> MASEVMNLSEEDIQFCQKAFSDYDEDGLGAIKVSDLKLALENIGCSLSENDLFKMISEVDEKNTGLIKFSDFLNIYYKQKYANLGDDDQDLVDAFVAMGGNADTTGSVDANRLIQIVKEEFEMTIDIVGL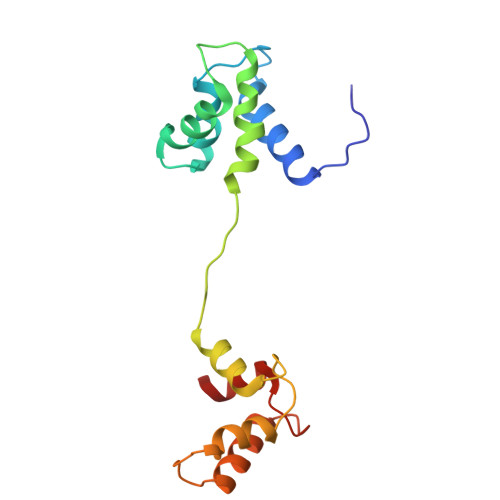IREIDKDGSGEIEYEEFKLL[3-(4-amino-6-methyl-1H-imidazo[4,5-c]pyridin-1-yl)azetidin-1-yl][1-({1-[(1R)-cyclohept-2-en-1-yl]piperidin-4-yl}methyl)-1H-pyrrol-3-yl]methanone 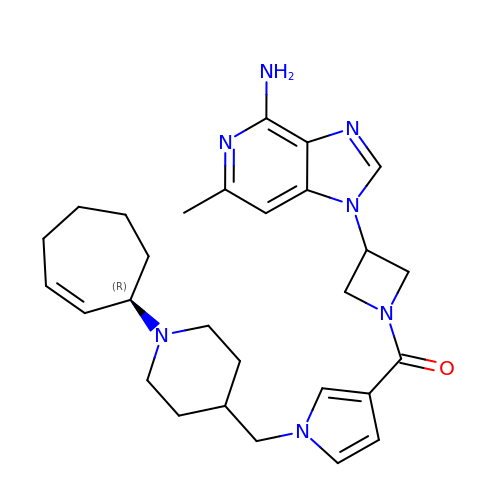| C28 H37 N7 O | HQHAEFHJXLPTMM-QHCPKHFHSA-N>[6x]MAEAKKGIDVILLYRVLKNEAKEAAWKMAFQTEHSNGKSRDADSTATKDGP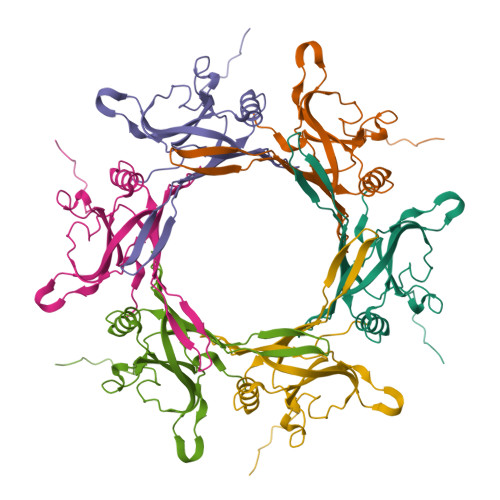IQNMAAIEYDFSATSIVAVGDKHIDELDDAFDNSELVEIWEIDKAEKGTDKDVDKYKATYFQGYVSSFSKTPNSEDALELEIEFAINGIGQKGYATLTTDQAEVVSYVFKDTVKVEEG>[12x]DKQWERFLVPYRQAVEELKVKLKGIRTLY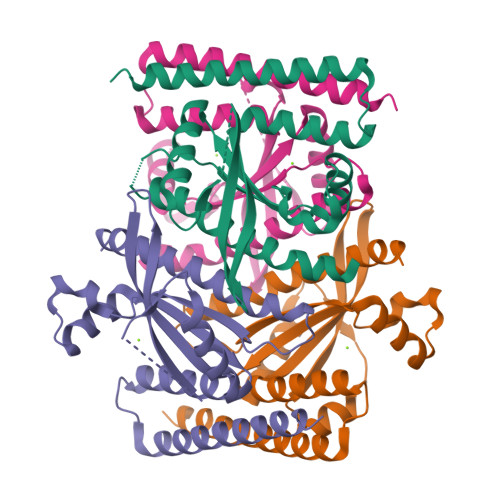EYEDDHSPIEFVTGRVKPVASILEKARRKSIPLHEIETMQDIAGLRIMCQFVDDIQIVKEMLFARKDFTVVDQRDYIAEHKESGYRSYHLVVLYPLQTVSGEKHVLVEIQIRTLAMNFWATIEHSLNYKYSGNIPEKVKLRLQRASEAASRLDEEMSEIRGEVQEAQAAFSRKKKGSEQQ> XIWIAQELRRRGDSFNAYY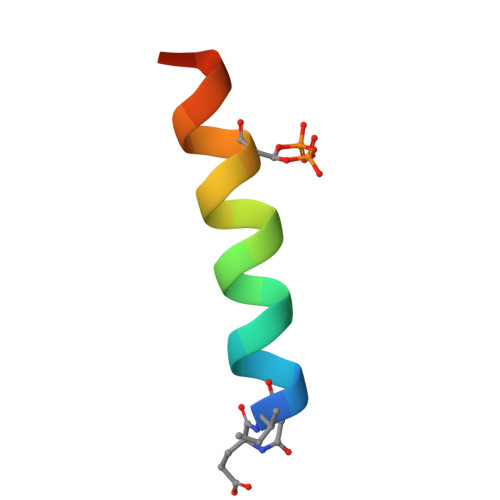AR>EAEATDPNGYIVFCPCMGRFGNQVDQFLGVLAFAKALDRTLVLPNFIEFKHPETKMIPFEFLFQVGTVAKYTRVVTMQEFTKKIMPTVWPPEKRKAFCWTPRQAIYDKSAEPGCHSKEGNPFGPYWDQIDVSFVGDEYFGDIPGGFDLNQMGSRKKWLEKFPSEEYPVLAFSSAPAPFPSKGKVWSIQKYLRWSSRITEQAKKFISANLAKPFVAVHLRNDADWVRVCEHIDTTTNRPLFASEQCLGEGHHLGTLTKEICSPSKQQILEQIVEKVGSIGAKSVFVASDKDHMIDEINEALKPYEIEAHRQEPDDMYTSLAIMGRADLFVGNCVSTFSHIVKRERDHAGQSPRPSAFFGIRAV[2x]

POFUT1 α-fucosylates serines or threonines present in EGF repeats containing the appropriate consensus sequence, C2-X(4-5)-[S/T]-C3, where C2 and C3 are the second and third conserved cysteines. In the present study we have solved the first crystal structure of CePOFUT1, which serves as a conserved family member. The protein shows a typical GT-B fold formed by two Rossmann domains. A cavity for GDP-fucose is localised in the interface between the domains and a contiguous solvent exposed pocket for EGF repeats was identified by electrostatic and docking studies.

To determine the structure of CePOFUT1 we obtained three different crystal forms. The fourth one is a crystal-form-III in complex with GDP, resembling a product complex. A comparison among the different crystal forms revealed minor conformational changes within the two domains (RMSD of 0.25 Å among apo crystal-form-I and soaked with GDP-fucose, and 0.66–0.86 Å among crystal-form-I compared to crystal-form-II and III, respectively) and some differences in order/disorder loop changes, such as a loop in the N-terminal domain (residues 125–134). The larger RMSD could have resulted from differences in crystal packing and not from bound ligands due to the small RMSD among crystals-form-I with and without the ligand. CePOFUT1 is a monomeric protein, as determined by gel filtration chromatography and confirmed by analytical ultracentrifugation (data not shown). Unlike Asp242 or Asp244, Arg240 played an important key role in binding and catalysis.>[2x]ETGETPPRFTRTPVDQTGVSGGVASFICQATGDPRPKIVWNKKGKKVSNQRFEVIEFDDGS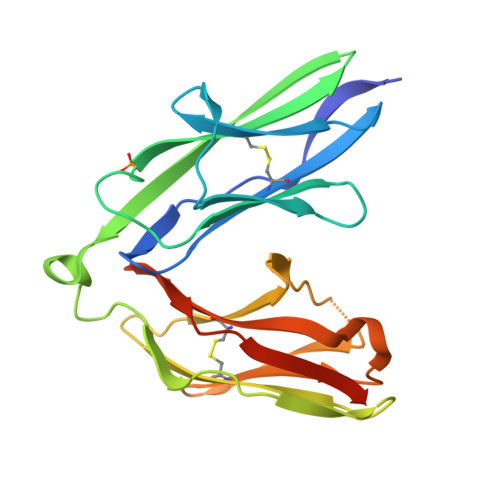GSVLRIQPLRTPRDEAIYECVASNNVGEISVSTRLTVLREDQIPRGFPTIDMGPQLKVVERTRTATMLCAASGNPDPEITWFKDFLPVDTSNNNGRIKQLRSESIGALQIEQSEESDQGKYECVATNSAGTRYSAPANLYVRGTKHHHHHH>MSLTENAERSLTDDRTLAENKERCLQMVAAWNRWELDGIIKYWAPDVVHYSEDKVVDTDEMIRRMEGGIQAFPDLHLDVKSIMAEEDRVILRITITATHKGRFGDLAPTNRKVAWHIVEELRFV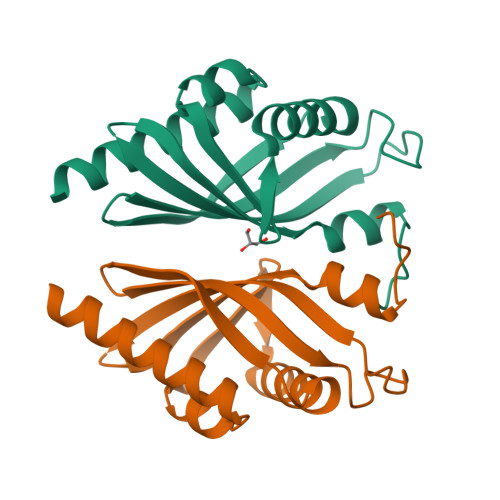DGKVVEHWDVMNYLPMLKELGKVPADV[2x]> INYKQLQLQERTNIRKCQELLEQLNGKINLTYRADFKIPMEMTEKMQ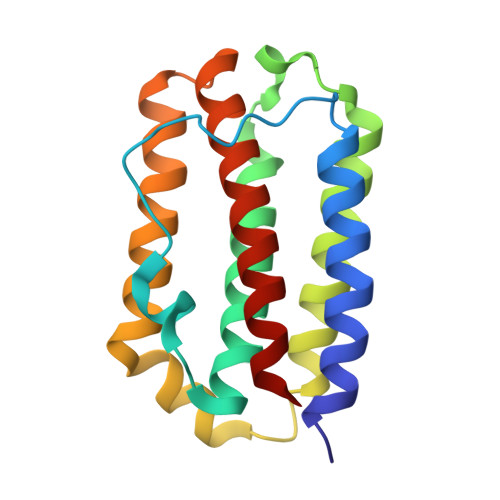KSYTAFAIQEMLQNVFLVFRNNFSSTGWNETIVVRLLDELHQQTVFLKTVLEEKQEERLTWEMSSTALHLKSYYWRVQRYLKLMKYNSYAWMVVRAEIFRNFLIIRRLTRNFQN>MNGAIKVGAWGGNGGSAFDMGPAYRIISVKIFSGDVVDGVDVTFTYYGKTETRHYGGSGGTPHEIVLQEG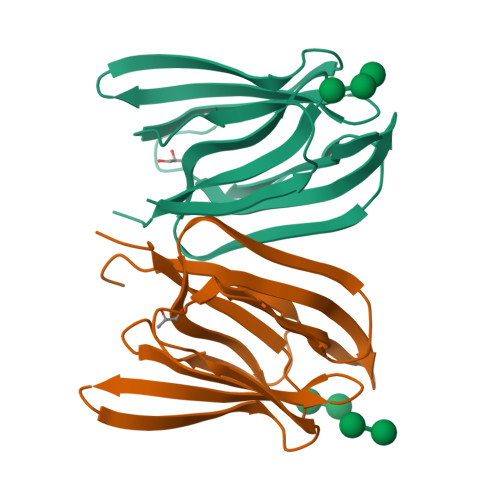EYLVGMAGEVANYTGAVVLGKLGFSTNKKAYGPFGNTGGTPFSLPIAAGKISGFFGRGGKFLDAIGVYLEPLEHHHHHH[4x]> GLSLMPWFHGKISGQEAVQQLQPPEDGLFLVRESARHPGDYVLCVSFGR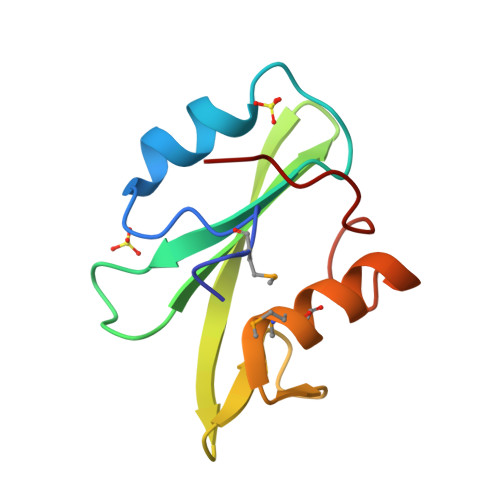DVIHYRVLHRDGHLTIDEAVFFCNLMDMVEHYSKDKGAICTKLVRPKRK>[4x]GAEDAGAFDKIQQIRAGDLNIGYVDIGPRDGQPVILLHGWPYDIQSYAQVAPALAQKGYRVIVPYLRGYGTTRFLSASTPRNGQPSAMAADIVHLMDALNIRQADLAGFDWGARTADIVAALWPQRVKSLVSVSGYLISSQQIGEKPLPPQAELSWWYQFYFATPRGEAGYRQNTHDFAKFIWHQASPQWQFSDATFAKTARALDNPDHVAITISNYRWRLG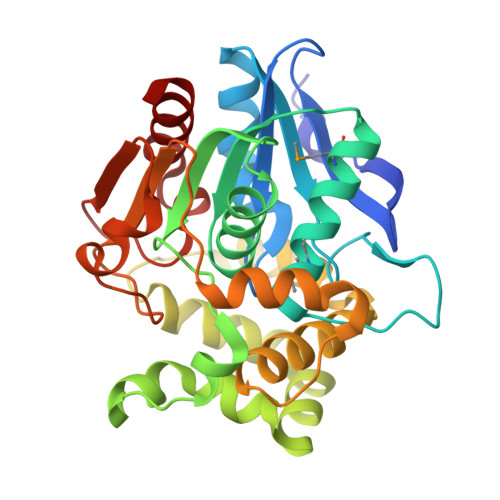LEKGEAKYAGYEQRLAALPPITVPTITLEGANNGAPHPAPASYRAKFTGKYEHRDLPGAVGHNPPQEDPTAFVQAVVDADRL> MNHLGKTEVFLNRFALRPLNPEELRPWRLEVVLDPPPGREEVYPLLAQVARRAGGVTVRMGDGLASWSPPEVLVLEGTLARMGQTYAYRLYPKGRRPLDPKDPGERSVLSALARRLLQERLRRLEGVWVEGLAVYRREHARGPGWRVLGGAVLDLWVSDSGAFLLEVDPAYRILCEMSLEAWLAQGHPLPKRVRNAYDRRTWELLRLGEEDPKELPLPGGLSLLDYHASKGRLQGREGGRVAWVADPKDPRKPIPHLTGLLVPVLTLEDLHEEEGSLALSLPWEERRRRTREIASWIGRRLGLGTPEAVRAQAYRLSIPKLMGRRAVSKPADALRVGFYRAQETALALLRLDGAQGWPEFLRRALLRAFGASGASLRLHTLHAHPSQGLAFREALRKAKEEGVQAVLVLTPPMAWEDRNRLKALLLREGLPSQILNVPLREEERHRWENALLGLLAKA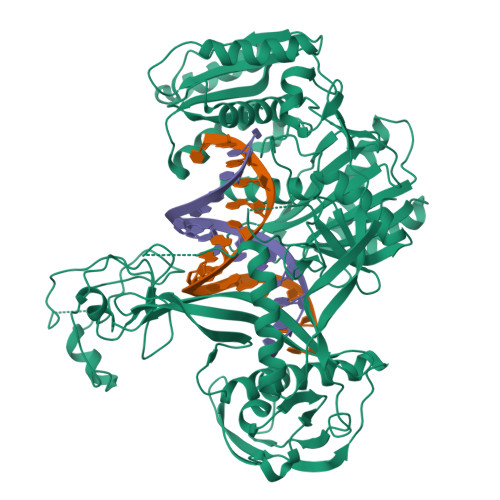GLQVVALSGAYPAELAVGFDAGGRESFRFGGAACAVGGDGGHLLWTLPEAQAGERIPQEVVWDLLEETLWAFRRKAGRLPSRVLLLREGRVPQDEFALALEALAREGIAYDLVSVRKSGGGRVYPVQGRLADGLYVPLEDKTFLLLTVHRDFRGTPRPLKLVHEAGDTPLEALAHQIFHLTRLYPASGFAFPRLPAPLHLADRLVKEVGRLGIRHLKEVDREKLFFV>GSHMASKISDNVRIKLYMEGTVNNHHFMCEAEGEGKPYEGTQMENIKVTKGGPLPFSFDILTPNCQLGSVAITKYTSGIPDYFKQSFPEGFTWERTTIYEDGAYLTTQQETKLDGNCLVYNIKILGCNFPPNGPVMQKKTQGWEPCCEMRYTRDGVLCGQTLMALKCADGNHLTCHLRTTYRSKK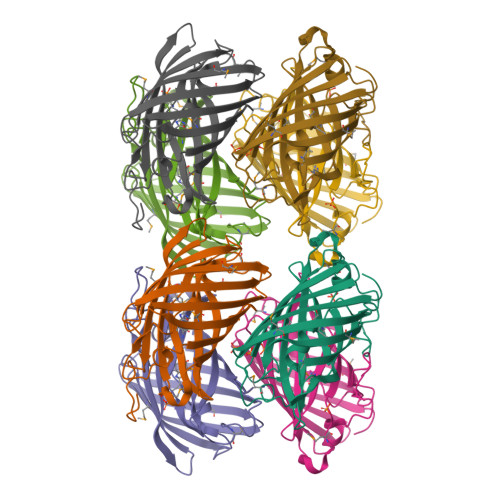AAKALQMPPFHFSDHRPEIVKVSENGTLFEQHESSVARYCQTCPSKLGHN[8x]> MLKAWHLPVAPFIKEQQERLMITLWLSGDDLPPRVTLRAEEDNEELSLPMHRLRQAPHPGVVAWRGEINLVNGQPRRRYSFKLLWADRQLWFTPQEFNRFPPARLEQFAVDLPDSGPQWVADQVFYQIFPDRFARSQSREAEQDATYYHHAAGHDIVRKAWDEPLTAEAGGSTFYGGDLDGISEKLPYLKQLGVTALYLNPVFVAPSVHKYDTEDYRRVDPQFGGDAALLRLRHNTQKE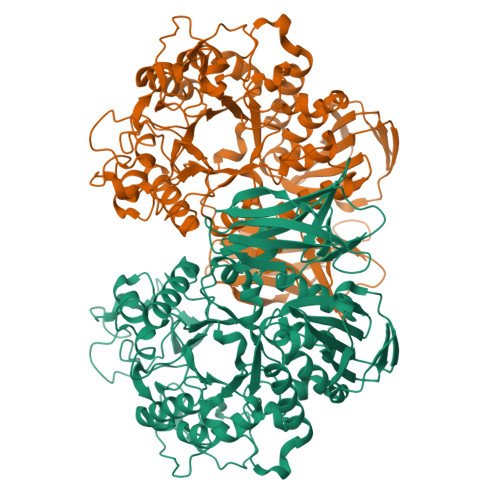GMRLILDGVFNHSGDSHAWFDRHQRGSGGACHNADSPWRDWYNFSPEGVAHDWLGYASLPKLDYRSSTLIDEIYGGEDSVVRHWLKAPWSMDGWRLDVVHMLGEGGGARNNLRHIAGITQAAKLERPDAFVFGEHFGDARQWLQADVEDSAMNYRGFTFPLWGFLANTDISYDPQKIDAQTCMAWMDNYRAGLSHQQQLRMFNQLDSHDTARFKSLLGKDVARLPLAVVWLFSWPGVPCIYYGDEVGVDGNNDPFCRKPFPWDPALQDGDLLDLYKRMSKLRKAHQALRYGGCQVIYAEDNVVVFVRVYKQQRVLVAINRGEACEVVIEDSPLLDVNGWQLKEGAGALHDGVLTLPAISASVWFSR>[2x]GSHMAPSRKFFVGGNWKMNGRKQSLGELIGTLNAAKVPADTEVV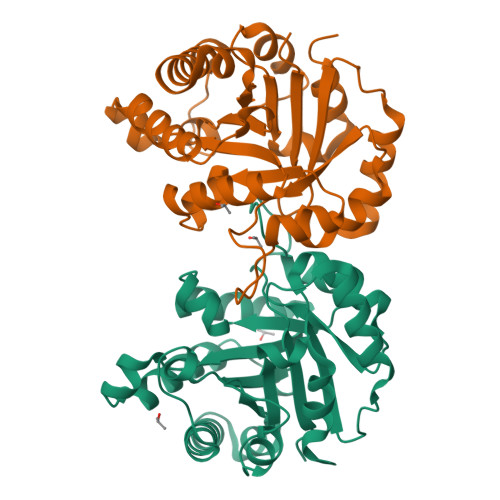CAPPTAYIDFARQKLDPKIAVAAQNCYKVTNGAFTGEISPGMIKDCGATWVVLGHSERRHVFGESDELIGQKVAHALAEGLGVIACIGEKLDEREAGITEKVVFEQTKVIADNVKDWSKVVLAYEPVWAIGTGKTATPQQAQEVHEKLRGWLKSNVSDAVAQSTRIIYGGSVTGATCKELASQPDVDGFLVGGASLKPELVDIINAKQ> MTTQAPTFTQPLQSVVVLEGSTATFEAHISGFPVPEVSWFRDGQVISTSTLPGVQISFSDGRAKLTIPAVTKANSGRYSLKATNGSGQATSTAELLVKAET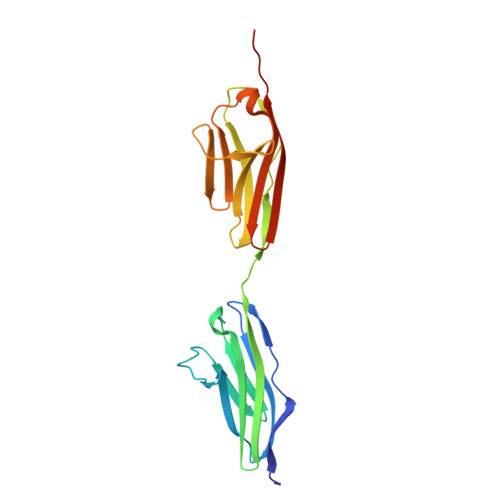APPNFVQRLQSMTVRQGSQVRLQVRVTGIPTPVVKFYRDGAEIQSSLDFQISQEGDLYSLLIAEAYPEDSGTYSVNATNSVGRATSTAELLVQGETREEF>MKTINSVDTKEFLNHQVANLN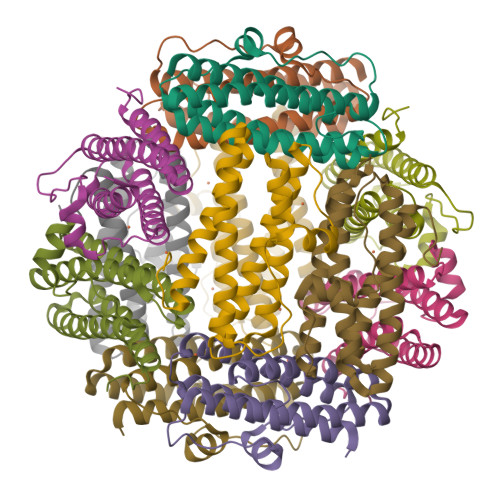VFTVKIHQIHWYMRGHNFFTLHEKMDDLYSEFGEQMDEVAERLLAIGGSPFSTLKEFLENASVEEAPYTKPKTMDQLMEDLVGTLELLRDEYQQGIELTDKEGDNVTNDMLIAFKASIDKHIWMFKAFLGKAPLE[24x]> GSMLKSKTFLKKTRAGGVMKIVREHYLRDDIGCGAPGCAACGGAHEGPALEPQPQDPASSVCPQPHYLLPDTNVLLHQIDVLEDPAIRNVIVLQTVLQEVRNRSAPVYKR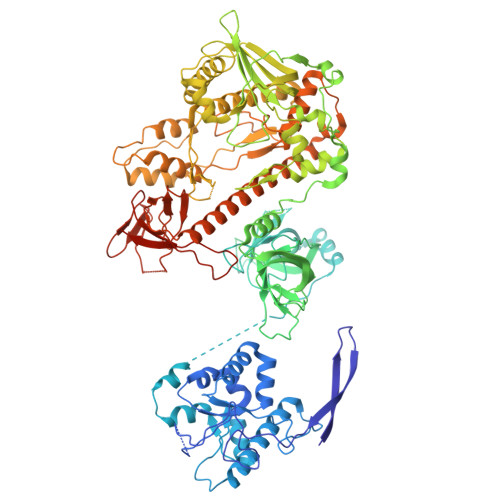IRDVTNNQEKHFYTFTNEHHRETYVEQEQGENANDRNNRAIRVAAKWYNEHLKKMSADNQLQVIFITNDRRNKEKAIEEGIPAFTCEEYVKSLTANPELIDRLACLSEEGNEIESGKIIFSEHLPLSKLQQGIKSGTYLQGTFRASRENYLEATVWIHGDSEENKEIILQGLKHLNRAVHEDIVAVELLPKSQWVAPSSVVLHDEGQNEEDVEKEEETERMLKTAVSEKMLKPTGRVVGIIKRNWRPYCGMLSKSDIKESRRHLFTPADKRIPRIRIETRQASTLEGRRIIVAIDGWPRNSRYPNGHFVRNLGDVGEKETETEVLLLEHDVPHQPFSQAVLSFLPKMPWSITEKDMKNREDLRHLCICSVDPPGCTDINDALHCRELENGNLEVGVHIADVSHFIRPGNALDQESARRGTTVYLCEKRIDMVPELLSSNLCSLKCDVDRLAFSCIWEMNHNAEILKTKFTKSVINSKASLTYAEAQLRIDSANMNDDITTSLRGLNKLAKILKKRRIEKGALTLSSPEVRFHMDSETHDPIDLQTKELRETNSMVEEFMLLANISVAKKIHEEFSEHALLRKHPAPPPSNYEILVKAARSRNLEIKTDTAKSLAESLDQAESPTFPYLNTLLRILATRCMMQAVYFCSGMDNDFHHYGLASPIYTHFTSPIRRYADVIVHRLLAVAIGADCTYPELTDKHKLADICKNLNFRHKMAQYAQRASVAFHTQLFFKSNGIVSEEAYILFVRKNAIVVLIPKYGLEGTVFFEEKDKPNPQLIYDDEIPSLKIEDTVFHVFDKVKVKIMLDSSNLQHQKIRMSLVEPQIPGISIPTDTSNMDLNGPKKKKMKLGK> MPGDHRRIRGPEESQPPQLYAADEEEAPGTRDPTRLRPVYARAGLLSQAKGSAY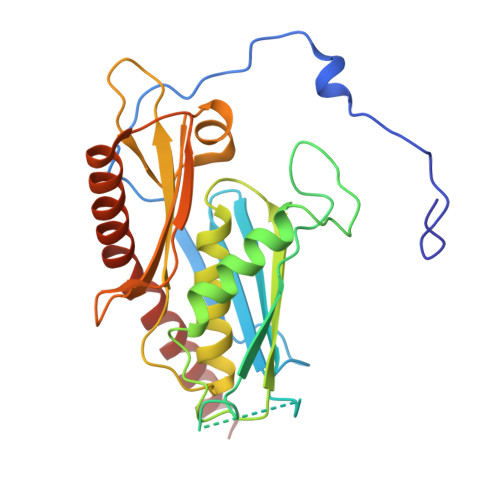LEAGGTKVLCAVSGPRQAEGGERGGGPAGAGGEAPAALRGRLLCDFRRAPFAGRRRRAPPGGCEERELALALQEALEPAVRLGRYPRAQLEVSALLLEDGGSALAAALTAAALALADAGVEMYDLVVGCGLSLAPGPAPTWLLDPTRLEEERAAAGLTVALMPVLNQVAGLLGSGEGGLTESWAEAVRLGLEGCQRLYPVLQQSLVRAARRRGAAAQP>GSQIHVDTMKVINDPIHGHIELHPLLVRIIDTPQFQRLRYIKQLGGGYYVFPGASHNRFEHSLGVGYLAGCLVHALGEKQPELQISERDVLCVQIAGLCHDLGHGPFSHMFDGRFIPLARPEVKWTHEQGSVMMFEHLINSNGIKPVMEQYGLIPEEDICFIKEQIVGPLESPVEDSLWPYKGRPENKSFLYEIVSNKRNGIDVDKWDYFARDCHHLGIQNNFDYKRFIKFARVCEVDNELRICARDKEVGNLYDMFHTRNSLHRRAYQHKVGNIIDTMITDAFLKADDYIEITGAGGKKYRISTAIDDMEAYTKLTDNIFLEILYSTDPKLKDAREILKQIEYRNLFKYVGETQPTGQIKIKREDYESLPKEVASAKPKVLLDVKLKAEDFIVDVINMDYGMQEKNPIDHVSFYCKTAPNRAIRITKNQVSQLLPEKFAEQLIRVYCKKVDRKSLYAARQYFVQWCADRNFTKPQDGDVIAPLITPQKKEWNDSTSVQNPTRLREASKSRVQLFKDDPM[16x]

Sterile alpha motif and HD domain-containing protein 1 (SAMHD1) is an important regulator of cellular 2′-deoxynucleoside-5′-triphosphate (dNTP) in mammalian cells. Although the HD-domain contains the active site, dNTP hydrolysis requires assembly of SAMHD1 into homo-tetramers. Here, sequences at the N and C termini of the HD-domain stabilise inter-monomer protein–protein interactions and incorporate four pairs of allosteric nucleotide-binding sites, AL1 and AL2, which regulate the enzyme through combined binding of G-based (AL1) and 2′-deoxynucleoside (AL2) triphosphates. Using combined biophysical and X-ray structural studies incorporating nucleotide analogues along with mutagenesis experiments we have now discovered that SAMHD1 uses a bi-metallic Fe–Mg centre to catalyse dNTP hydrolysis in a reaction similar to those catalysed by HD domains in both human and bacterial phosphodiesterase PDE enzymes.

In addition, we determined the structures of two co-complexes of wt-SAMHD1(109-626), also in the presence of Mg2+, with (i) GTP (AL1), dATP (AL2) and dCMPNPP (active site) and (ii) GTP (AL1), dATP (AL2) and TMPNPP (active site). dATP was added to the latter two complexes to stimulate tetramer assembly, as dCMPNPP and TMPNPP are poor AL2 activators. Further investigation using inhibition assays revealed that all dNMPNPP analogues were actually competitive inhibitors of SAMHD1-dNTP triphosphohydrolase activity, with inhibition constants (Ki) ranging from 0.78 µM for dAMPNPP to 0.052 µM for dGMPNPP, with the following rank order of increasing affinity: dAMPNPP < TMPNPP < dCMPNPP < dGMPNPP. The resolution of these structures varied between 2.0 and 3.2 Å, but all structures contain highly homologous “closed” tetramers of the SAMHD1 catalytic domain, with pairwise root-mean-square deviations (RMSDs) of <0.5 Å across all atoms in each tetramer. In the active site of the dNMPNPP structures, regardless of the nucleotide base, it is apparent that the side chain of Asp311 of the HD motif not only makes a coordinate bond with the bound active site Fe but also acts as an acceptor in a hydrogen bonding interaction with the proton (Himido) of the α,β-imido group of the dNMPNPP.The majority of traits controlled by rhl transcription factor RhlR depend on PqsE, a dispensable thioesterase in Pseudomonas Quinolone Signal (PQS) biosynthesis that interferes with RhlR through an enigmatic mechanism likely involving direct interaction of both proteins. Here we show that PqsE and RhlR form a 2:2 protein complex that, together with RhlR agonist N-butanoyl-L-homoserine lactone (C4-HSL), solubilizes RhlR and thereby renders the otherwise insoluble transcription factor active. PqsE is a thioesterase that triggers transcription of the RhlR regulon through a hitherto cryptic mechanism, which we identify here as involving a significant chaperone-like component that enhances the stability of RhlR via protein complex formation. In common with many other gram-negative bacteria, two QS circuits use N-acyl-L-homoserine lactones (HSLs) as autoinducers, namely N-(3-oxododecanoyl)-L-HSL (3-oxo-C12-HSL) and N-butanoyl-L-HSL (C4-HSL), which are produced by autoinducer synthases LasI and RhlI and activate the LuxR-type transcription factors LasR and RhlR, respectively.

We, therefore, investigated whether both proteins engage in a complex when affinity-tagged variants are co-expressed in E. coli. This was indeed the case but required the presence of the cognate autoinducer C4-HSL or of the synthetic RhlR ligand mBTL. The PqsE segment adopted the same dimeric configuration as in the free protein but with a slightly twisted arrangement. The RhlR sequence displayed the expected homodimeric structure of a LuxR-type transcription factor and C4-HSL as well as mBTL were found in the anticipated ligand binding site (Supplementary Fig. 4a/b). The acyl chain of C4-HSL points into a hydrophobic pocket of the ligand binding site in RhlR, again with high similarity to related structures. This pocket extends beyond the butyryl group of C4-HSL and is not fully closed towards the solvent, explaining why ligands such as mBTL can be accommodated without obvious changes to the structure and suggesting that RhlR could sense other HSLs as well. The butanol-m-bromophenol group of mBTL resides in the hydrophobic acyl-binding tunnel leading towards the lactone binding site, and the m-bromophenol establishes π-stacking interactions with Y64 and Y72, two residues also contained in wildtype RhlR. The synthetic HSL analogue mBTL has been developed as a RhlR antagonist, however, using pyocyanin production as a proxy for RhlR/PqsE-mediated quorum sensing, we observed that mBTL induced similar levels of pyocyanin as exogenously supplied C4-HSL in a ΔrhlI mutant of P. aeruginosa PA14, suggesting again that stabilization is a key factor of RhlR-mediated signaling.

>MGHHHHHHAENLYFQGHMLRLSAPGQLDDDLCLLGDVQVPVFLLRLGEASWALVEGGISRDAELVWADLCRWVADPSQVHYWLITHKHYDHCGLLPYLCPRLPNVQVLASERTCQAWKSESAVRVVERLNRQLLRAEQRLPEACAWDALPVRAVADGEWLELGPRHRLQVIEAHGHSDDHVVFYDVRRRRLFCGDALGEFDEAEGVWRPLVFDDMEAYLESLERLQRLPTLLQLIPGHGGLLRGRLAADGAESAYTECLRLCRRLLWRQSMGESLDELSEELHRAWGGQSVDFLPGELHLGSMRRMLEILSRQALPLD[2x];>[2x]MRNDGGFLLWWDGLRSEMQPIHDSQGVFAVLEKEVRRLGFDYYAYGVRHTIPFTRPKTEVHGTYPKAWLERYQMQNYGAVDPAILNGLRSSEMVVWSDSLFDQSRMLWNEARDWGLCVGATLPIRAPNNLLSVLSVARDQQNISSFEREEIRLRLRCMIELLTQKLTDLEHPMLMSNPVCLSHREREILQWTADGKSSGEIAIILSISESTVNFHHKNIQKKFDAPNKTLAAAYAAALGLI>MENFTTNLNQLARVGGIDPLIGREKELERAIQVLCRRRKNNPLLVGESGVGKTAIAEGLAWRIVQGDVPEVMADCTIYSLDIGSL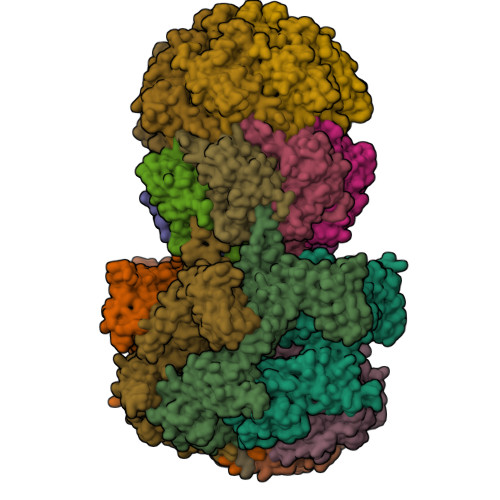LAGTKYRGDFEKRFKALLKQLEQDTNSILFIDEIHTIIGAGAASGGQVDAANLIKPLLSSGKIRVIGSTTYQEFSNIFEKDRALARRFQKIDITEPSIEETVQIINGLKPKYEAHHDVRYTAKAVRAAVELAVKYINDRHLPDKAIDVIDEAGARARLMPVSKRKKTVNVADIESVVARIARIPEKSVSQSDRDTLKNLGDRLKMLVFGQDKAIEALTEAIKMARAGLGHEHKPVGSFLFAGPTGVGKTEVTVQLSKALGIELLRFDMSEYMERHTVSRLIGAPPGYVGFDQGGLLTDAVIKHPHAVLLLDEIEKAHPDVFNILLQVMDNGTLTDNNGRKADFRNVVLVMTTNAGVRETERKSIGLIHQDNSTDAMEEIKKIFTPEFRNRLDNIIWFDHLSTDVIHQVVDKFIVELQVQLDQKGVSLEVSQEARNWLAEKGYDRAMGARPMARVIQDNLKKPLANELLFGSLVDGGQVTVALDKEKNELTYGF[6x];>[14x]ALVPMVIEQTSRGERSFDIYSRLLKERVIFLTGQVEDHMANLIVAQMLFLEAENPEKDIYLYINSPGGVITAGMSIYDTMQFIKPDVSTICMGQAASMGAFLLTAGAKGKRFCLPNSRVMIHQPLGGYQGQATDIEIHAREILKVKGRMNELMALHTGQSLEQIERDTERDRFLSAPEAVEYGLVDSILTHR> MAHFRYYKLAVQPQVNKEIKNNNDVDIDKTLVAKQSVVKFQLKTADLPAGRAKTTSFVLVDPLPSGYQFNLEATKAASPGFDVSYDKATNTVTFKATAATLATFNADLTKSVATIYPTVVGQVLNDGATYKNNFTLTVNDAYGIKSNVVRVTTPGKPNDPDNPNNNYIKPTKVNKNENGVVIDGKTVLAGSTNYYELTWDLDQYKNDRSSADTIQKGFYYVDDYPEEALELRQDLVKITDANGNKVTGVSVDHYTSLEAAPQEVRDVLSKAGIRPKGAFQIFRADNPREFYDTYVKNGIDLKIVSPMVVKKQMGQTGGSYENQAYQIDFGNGYASNIVINNVPKINPKKDVTLTLDPADTNNVDGQTIPLNTVFNYRLIGGIIPADHSEELFEYNFYDDYDQTGDRYTGQYKVFAKVDITLKDGSVIKSGTDLTQHTTAEVDATKGALTIKFKEDFLRSVSIDSAFQAESYIQMKRIAAGTFENTYVNTV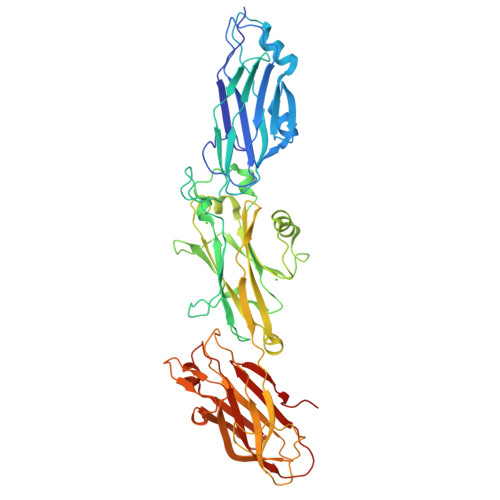NKVAYASENLYFQGLEHHHHHH>GSHMISEHDSVLEKYPRIQKVLNSTVPALSLNSSTRYEGKIINIGGTIIKARLPKARIGAFYKIEPSQRLAEVIAIDEDEVFLLPFEHVSGMYCGQWLSYQGDEFKIRVGDALLGRLIDGIGRPMESNIVAPYLPFERSLYAEPPDPLLRQVIDQPFILGVRAIDGLLTCGIGQRIGIFAGSGVGKSTLLGMICNGASADIIVLALIGERGREVNEFLALLPQSTLSKCVLVVTTSDRPALERMKAAFTATTIAEYFRDQGKNVLLMMDSVTRYARAARDVGLASGEPDVRGGFPPSVFSSLPKLLERAGPAPKGSITAIYTVLLESDNVNDPIG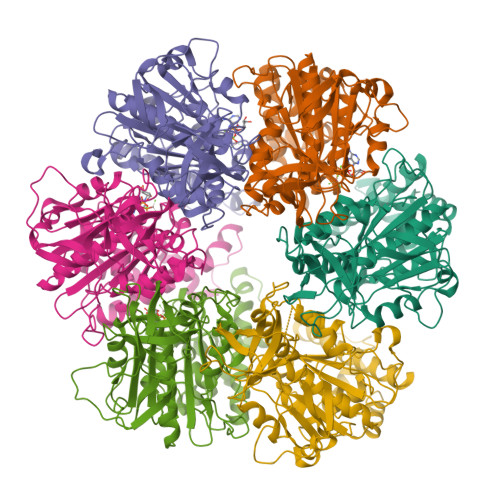DEVRSILDGHIVLTRELAEENHFPAIDIGLSASRVMHNVVTSEHLRAAAECKKLIATYKNVELLIRIGEYTMGQDPEADKAIKNRKLIQNFIQQSTKDISSYEKTIESLFKVVA[6x]>MSLRSGQLFRFLAVPLAIALMLGSMPGIGTSKAYAYTASDGDTAMKAFNDTFWDPNAKMFWKDSKREKHQDFWVEAELWELVMDAYQHTSDPALKAELKTQIDDVYDGTVAKYGQDWTNNPFNDDIMWWAMGSARAYQITGNPRYLEAARDHFDFVYDTQWDEEFANGGIWWLNSDHNTKNACINFPAAQAALYLYDITKDEHYLNAATKIFRWGKTMLTDGNGKVFDRIEIEHGAVPDATHYNQGTYIGSAVGLYKATGNAVYLDDAVKAAKFTKNHLVDSNGVLNYEGPNGDLKGGKTILMRNLAHLQKTLDETGQYPEFSAEFDEWLAFNIEMAWSHQNSDHIVDGNWAGQLLSGTYESWSSAAAVQAL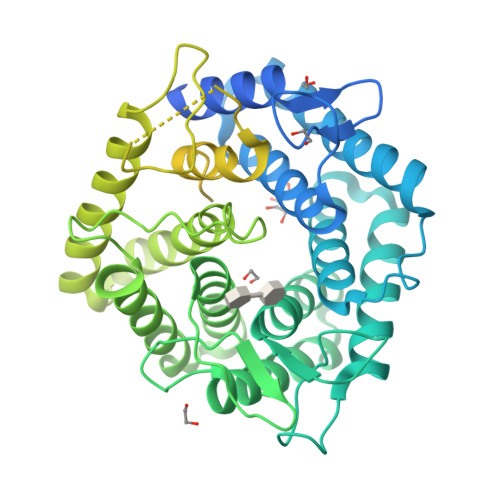NGIKPMEAELHYGVKNPFDKIEAERYNIGSGFVLEGAFEGSLQLGGIQHGSYAAYKNVDFGSDGAIGFIARASSGTGGGNIEIRLDSKDGPKVGTLNVEGTGDWNQYIDAVTLLKDDQGAPSTITGVHDVYLVFTKTNDDYLFNLNWVKFTTTDPTETDAYAKLKAGNYDSSEGLSKHAEFGYLDAIHHNAYASYEGIDFGSINRRHLRAPWQHRGR[2x]> VNQSETEIEILAEKIARWARARSAEIERDRRLPDELVTRLREAGLLRATMPREVAAPELAPGRALRCAEAVARGDASAGWCVSIAITSALLVAYLPARSREEMFGGGRGVAAGVWAPRGTARSVDGGVVVSGRWPFCSGINHADIMFAGCFVDDRQVPSVVALNKDELQVLDTWHTLGLRGTGSHDCVADDVFVPADRVFSVFDGPIVDRPLYRFPVFGFFALSIGAAALGNARAAIDDLVELAGGKKGLGTTRTLAERSATQAAAATAESALGAARALFYEVIEAAWQVSHDAEAVPVTMRNRLRLAATHAVRTSADVVRSMYDLAGGTAIYDNAPLQRRFRDAFTATAHFQVNEASRELPGRVLLDQPADVSML

Our subsequent investigation of one gene cluster (Rv3093c-Rv3095) associated with ethionamide resistance that contained a putative monooxygenase/repressor pair with some resemblance to ethA/ethR, indicates that Rv3094c is likely a flavin-dependent monooxygenase that sulfoxygenates ethionamide, and Rv3095 is its transcriptional regulator. Ethionamide is a second-line anti-tubercular drug used to treat patients infected with multi-drug-resistant or extensively drug-resistant isolates, and is a pro-drug that requires metabolic activation before it can exert its cytotoxic effects. To investigate the mechanism of ethionamide sulfoxygenation by Rv3094c, we solved protein crystal structures of apo-Rv3094c, and Rv3094c in complex with FMN (Rv3094c-FMN) and ethionamide (Rv3094c-FMN-ETH), at resolutions of 1.91 Å, 2.00 Å, and 1.64 Å, respectively. All three crystals contained one tetramer per asymmetric unit, tetramers being formed by two homodimers, the C-terminal domain primarily mediating interactions between the two monomers.

Superposition of apo-Rv3094c structural homologs not only reveals strong structural conservation of overall topology, but confirms that the location of the FMN binding site, lying in the pocket between the β-sheet and the C-terminal domain, and stabilization of the flavin ring by hydrogen bonds are also conserved. Ethionamide is embedded within a hydrophobic pocket comprised of the β-barrel domain and the C-terminal helix domain and is surrounded by the hydrophobic side chains of W115, P117, P158, V202, F218, F352, Q353, and M375. To evaluate which amino acids are important in interactions between Rv3094c and FAD and/or ethionamide, we constructed mutants based on the structure of the Rv3094c-FMN-ETH complex. ETH-SO synthesis was markedly altered by mutation of either of the two residues involved in both the FAD and ethionamide pockets (F352 and W115) or those specific to the FAD (W80, S138, W174, L179, and H351) or ethionamide (P117 and V202) pockets, indicating that these residues are all important in FAD/ethionamide binding. Mutation of W115 and P117 to arginine (R) (changing the hydrophobic side chain into a hydrophilic side chain with an additional 3-carbon aliphatic straight chain) blocked ethionamide activation more notably than when these residues were mutated to alanine (A) (simply removing the large side chain). In the structure of p-Hydroxyphenylacetate (HPA) hydroxylase, a structural and functional homolog of Rv3094c, HPA passes through a gate formed by F266 to interact with FMNH-.The E.coli Fic protein EcFicT forms a tight complex with its cognate antitoxin EcFicA. EcFicT adopts the conserved Fic fold, but with a distinct active site signature motif and an additional hydrophobic binding pocket in the vicinity of the active site loop. EcFicA forms two parallel α-helices that tightly embrace EcFicT. According to this classification, EcFicT belongs to class I with the inhibitory helix provided by EcFicA, a small protein coded immediately upstream of the ecficT gene.

The G55R mutation encoded by the fic-1 allele caused cell filamentation at non-permissive temperature (43°C) in the presence of high concentration of cAMP (1.5 mM) in the culture medium. However, the EcFicTG55R mutant in complex with EcFicA (EcFicTG55RA) yielded crystals that diffracted to 2.0 Å. The best solution (TFZ = 11.6 and LLG = 206) was obtained in space group P65 yielding two EcFicT molecules in the asymmetric unit. Our crystal structures show that the G55R mutation encoded by the fic-1 allele, which results in the cell filamentation phenotype, does not affect the structure of EcFicT. The arginine 55 side-chain forms a salt-bridge with glutamate 107 of helix α3, which is conserved in EcFicT-like homologs. One could speculate that the glycine to arginine mutation may reduce the main-chain flexibility. However, despite the additional salt-bridge, the G55R variant is not more stable than the wild-type protein, as has been shown above by DSF. The EcFicTG55RA crystal structure revealed that the site of mutation is neither close to the presumed active site nor the presumed target recognition site. Also in EcFicTG55RA, such an intermolecular salt-bridge is observed (E28–R146). In EcFicTG55RA, the flap is stabilized by crystal contacts and is fully ordered. In the EcFicTG55RA structure, the base-binding pocket is nevertheless partly restricted by the conformation that adopts the glutamine 84 of EcFicT located at the tip of the flap.

>[2x]MGSSHHHHHHSQDPNSSSARLQVEMGDKFGEGRDPYLYPGLDIMRNRLNIHQQQRLEQAAYEMTALRAATIELGPLVRRLPHLRTIHRQLYQDIFDWAGQLREVDIYQGDTPFCHFAYIEKEGNALMQDLEEEGYLVGLEKAKFVERLAHYYCEINVLHPFRVGSGLAQRIFFEQLAIHAGYQLSWQGIEKEAWNQANQSGAMGDLTALQMIFSKVVSEAGESE;>MAYPYDVPDYAAAVKKLTDKQKSRLWELQRNRNFQASRRLEGVEMPLVTLTAAEALARLEELRSHYER[2x]>MTNLQTFEL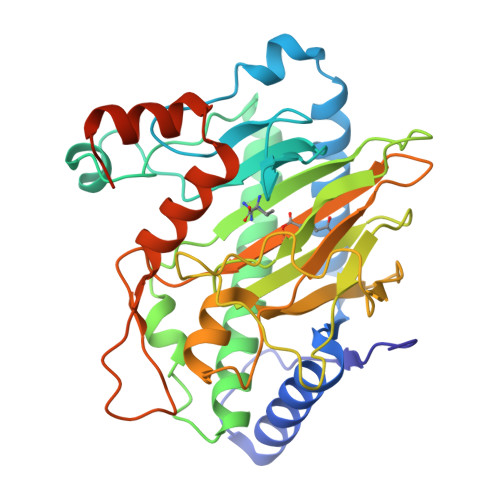PTEVTGCAADISLGRALIQAWQKDGIFQIKTDSEQDRKTQEAMAASKQFCKEPLTFKSSCVSDLTYSGYVASGEEVTAGKPDFPEIFTVCKDLSVGDQRVKAGWPCHGPVPWPNNTYQKSMKTFMEELGLAGERLLKLTALGFELPINTFTDLTRDGWHHMRVLRFPPQTSTLSRGIGAHTDYGLLVIAAQDDVGGLYIRPPVEGEKRNRNWLPGESSAGMFEHDEPWTFVTPTPGVWTVFPGDILQFMTGGQLLSTPHKVKLNTRERFACAYFHEPNFEASAYPLFEPSANERIHYGEHFTNMFMRCYPDRITTQRINKENRLAHLEDLKKYSDTRATGS[4x]> MALKTKPRWDKYDGYVGNYRGVLGEDIDLDTEANRVLAVGTNSNGAIVVGAGQTGIKGL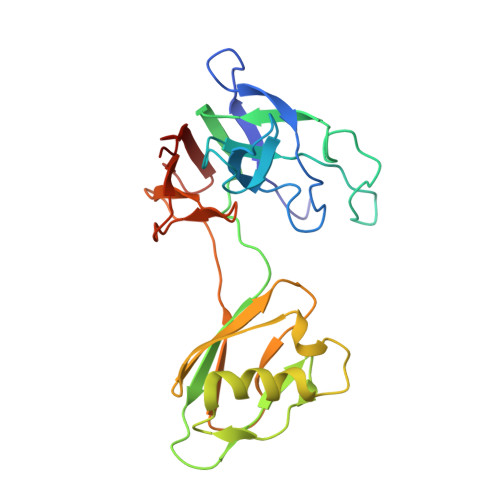MIVAVGADIHGAMLDGGINNHAGDPQDVGKHGEITNFQPTVFGRTFGVAISATEGNVKLAVNGVDTGNIAYDTSAANLKSGIVAVDDGFTADDFTVTGTAPNFTIVTTRTDVTITASGEGVTVTEATSVAAAGTNYYGHADGTVNAVKGSDGVYVGHTQEADRLIVNVKDEED>[7x]APSLLHKYMGIFFSTMSSEELLGSLDSFDAREDDIFLVSYPKSGTHWLAEVIERIPDAGITLTSPIELGDISKFEELKRIPKRRAIPTHLNYEMLPVTVKQKQCKIIYIVRNPKDTAVSM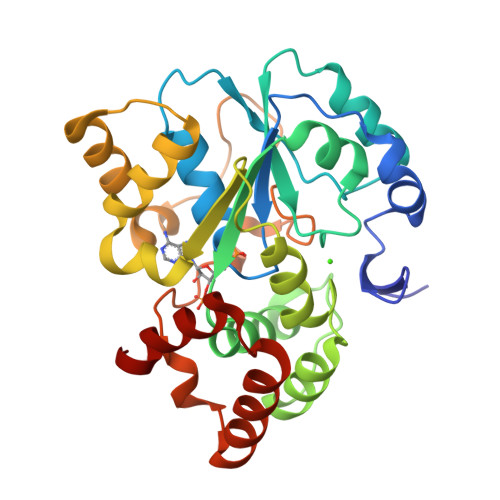FHYYRDNPNLPSTETWAAFLELFLKGDVVYGSWFDHVLSWEEHKNDKNVLFIFYEEMKKDFVKSLKKITAFLGIDVNDSEMAKIARSTSFSEMKSNAAKENCDPNHVICALTSDRNLVFRKGVVGDWINYFTPKQNRGFDELFTEKMRNSDVGRCLKEYAHSA;> AILHKYMGIFFSTMSSEELLGSLDSFDAREDDIFLVSYPKSGTHWLAEVIERIPDAGITLTSPIELGDISKFEELKRIPKRRAIPTHLNYEMLPVTVKQKQCKIIYIVRNPKDTAVSMFHYYRDNPNLPSTETWAAFLELFLKGDVVYGSWFDHVLSWEEHKNDKNVLFIFYEEMKKDFVKSLKKITAFLGIDVNDSEMAKIARSTSFSEMKSNAAKENCDPNHVICALTSDRNLVFRKGVVGDWINYFTPKQNRGFDELFTEKMRNSDVGRCLKEYAHSA;>[4x]PSLLHKYMGIFFSTMSSEELLGSLDSFDAREDDIFLVSYPKSGTHWLAEVIERIPDAGITLTSPIELGDISKFEELKRIPKRRAIPTHLNYEMLPVTVKQKQCKIIYIVRNPKDTAVSMFHYYRDNPNLPSTETWAAFLELFLKGDVVYGSWFDHVLSWEEHKNDKNVLFIFYEEMKKDFVKSLKKITAFLGIDVNDSEMAKIARSTSFSEMKSNAAKENCDPNHVICALTSDRNLVFRKGVVGDWINYFTPKQNRGFDELFTEKMRNSDVGRCLKEYAHSA>[4x]DNILYSGETLSTGEFLNYGSFVFIM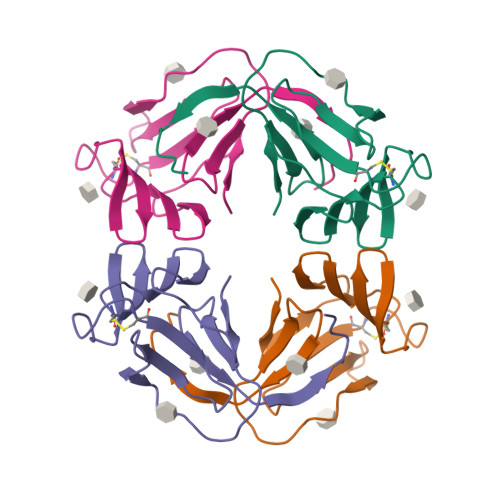QEDCNLVLYDVDKPIWATNTGGLSRSCFLSMQTDGNLVVYNPSNKPIWASNTGGQNGNYVCILQKDRNVVIYGTDRWATGTHTG> SGSREPNLFRSLVGTSRAIQQVRQMMQQVADTDASVLILGESGTGKEVVARNLHYHSKRREGPFVPVNCGAIPAELLESELFGHEKGAFTGAITSRAGRFELANGGTLFLDEIGDMPLPMQVKLLRVLQERTFERVGSNKTQNVDVRIIAATHKNLEKMIEDGTFREDLYYRLNVFPIEMAPLRERVEDIALLLNELISRMEHEKRGSIRFNSAAIMSLCRHDWPGNVRELANLV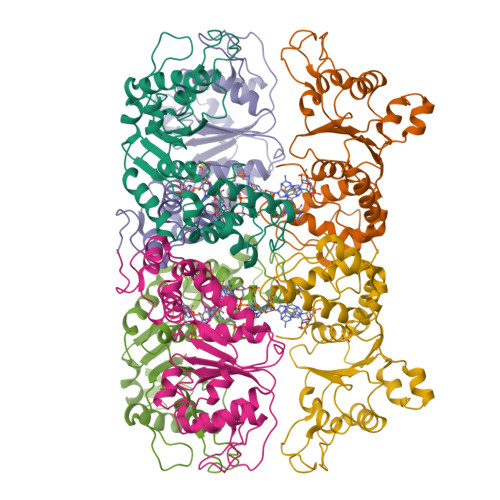ERLAIMHPYGVIGVGELPKKFRHVDDEDEQLASSLREELEERAAINAGLPGMDAPAMLPAEGLDLKDYLANLEQGLIQQALDDAGGVVARAAERLRIRRTTLVEKMRK>[12x]MAHHHHHHGTEKTPDDVFKLAKDEKVEYVDVRFCDLPGIMQHFTIPASAFDKSVFDDGLAFDGSSIRGFQSIHESDMLLLPDPETARIDP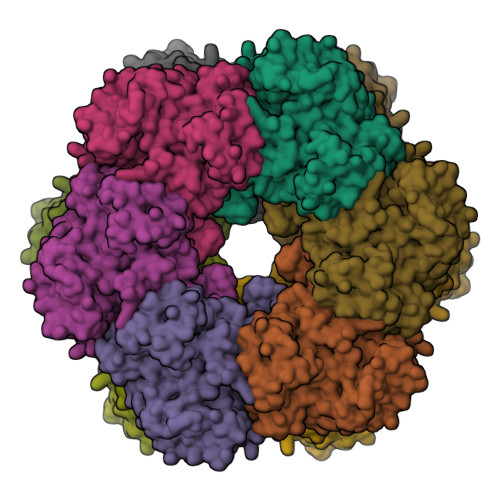FRAAKTLNINFFVHDPFTLEPYSRDPRNIARKAENYLISTGIADTAYFGAEAEFYIFDSVSFDSRANGSFYEVDAISGWWNTGAATEADGSPNRGYKVRHKGGYFPVAPNDQYVDLRDKMLTNLINSGFILEKGHHEVGSGGQAEINYQFNSLLHAADDMQLYKYIIKNTAWQNGKTVTFMPKPLFGDNGSGMHCHQSLWKDGAPLMYDETGYAGLSDTARHYIGGLLHHAPSLLAFTNPTVNSYKRLVPGYEAPINLVYSQRNRSACVRIPITGSNPKAKRLEFRSPDSSGNPYLAFSAMLMAGLDGIKNKIEPQAPVDKDLYELPPEEAASIPQTPTQLSDVIDRLEADHEYLTEGGVFTNDLIETWISFKRENEIEPVNIRPHPYEFALYYDV>[2x]MI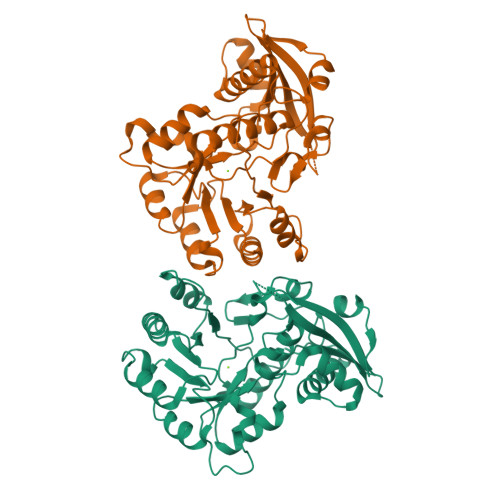KISYSPYTLKPVQSLNAATAATAREGVLLKVEWNDGLYGFADLHPWPELGDLSLEEQLSDLRMGRMTTQIEQSIWLARRDALLRKEKKHVFDGGEKIKNNYLLSHFQDLKPGFLDGLKNEGYNTVKVKMGRDLQKEADMLTHIAASGMRMRLDFNALGSWQTFEKFMVNLPLTVRPLIEYVEDPFPFDFHAWGEARKLAKIALDNQYDKVPWGKIASAPFDVIVIKPAKTDVDKAVAQCQKWNLKLAVTSYMDHPVGVVHAVGVAMELKDKYGDMILESGCLTHRLYQMDSFAAELSTQGPYLLKNKGTGVGFDKLLEALTWYQLKVR> SEFVPPPECPVFEPSWEEFTDPLSFIGRIRPLAEKTGICKIRPPKDWQPPFACEVKSFRFTPRVQRLNELEAMTRVRLDFLDQLAKFWELQGSTLKIPVVERKILDLYALSKIVASKGGFEMVTKEKKWSKVGSRLGYLPGKGTGSLLKSHYERILYPYELFQSGVSLMGVQMPNLDLKEKVEPEVLSTDTQTSPEPGTRMNILPKRTRRVKTQSESGDVSRNTELKKLQIFGAGPKVVGLAMGTKDKEDEVTRRRKVTNRSDAFNMQMRQRKGTLSVNFVDLYVCMFCGRGNNEDKLLLCDGCDDSYHTFCLIPPLPDVPKGDWRCPKCVAEECSKPREAFG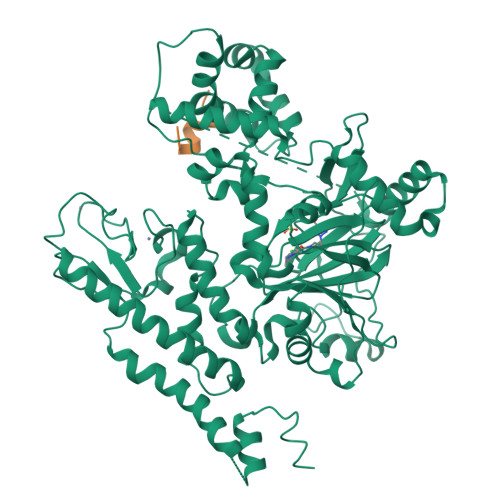FEQAVREYTLQSFGEMADNFKSDYFNMPVHMVPTELVEKEFWRLVSSIEEDVIVEYGADISSKDFGSGFPVKDGRRKILPEEEEYALSGWNLNNMPVLEQSVLAHINVDISGMKVPWLYVGMCFSSFCWHIEDHWSYSINYLHWGEPKTWYGVPSHAAEQLEEVMRELAPELFESQPDLLHQLVTIMNPNVLMEHGVPVYRTNQCAGEFVVTFPRAYHSGFNQGYNFAEAVNFCTADWLPIGRQCVNHYRRLRRHCVFSHEELIFKMAADPECLDVGLAAMVCKELTLMTEEETRLRESVVQMGVLMSEEEVFELVPDDERQCSACRTTCFLSALTCSCNPERLVCLYHPTDLCPCPMQKKCLRYRYPLEDLPSLLYGVKVRAQSYDTWVSRVTEALSANFNHKKDLIELRVMLEDAEDRKYPENDLFRKLRDAVKEAETCASVGNS> MQKMLYFDDDVKQIVDHMFFKGFMFNDERIDRYFKESFTLRFLYREIGRQTVESFASQVLYITMTHEDYIYRVYGSDMYKYIEQVTDTQSQDLGKAIENAIEQGQTKDRQQDKGHEEYKDYEDTITKSFDDNRTAESTLPQSKVNIDVDNTVLDYADTNTISRDKNTSETVSEKTGTKDNTFDSLRNGESDTKRNTQSQNEMNRTGLTKQYLIDNLQKLYSMRDTIFK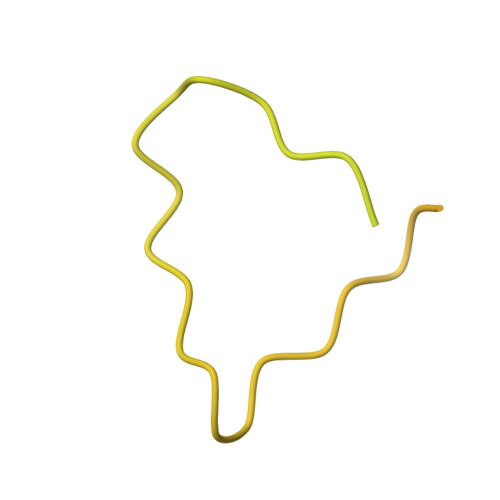TYDKECFLHIW>[2x]VTTTATLTYPFHDWSQELSPRYAQLRASDAPVCPVVSEGT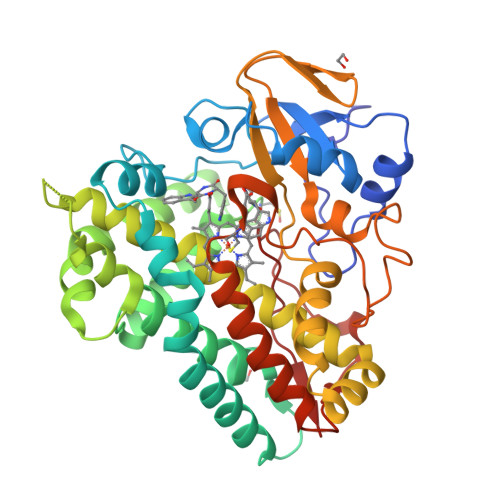GDPLWLVTRYATAVKLLEDSRFSSEAAQASGAPRQEPVELRAPGTRGDAIAMLREAGLRSVLADGLGPRAVRRHQGWINDLAETLMSELASREGTFDLAADFVEPLSSALVSRTLLGELSADERDLLAHCADTGLRFCGVTHEEQVHAFTQMHEFFLEHARRLAGTPGEHLLKLIAEAPVDQGPLSDEALAEAGSLLVVAGFPTSSGFLCGALLTLLRHPDAVQELHAHPERVPSAVEELLRYTPLSTGSVKRMATEDLEIDGVRIKAGEVVMVSLEAVNHDPDAFEDPDVFRPGREGPMHFGFGRGRHFCPGNRLARCVIEATVRAVARRPGLRLAVAPEEISWHEGLFFRRPRAIPATW>MSQSQRSTADWQRLDAAHHLHPFTDYGELNTKGSRIITRAEGCYLWDSDGNQILDGMAGLWCVNIGYGRKELAEVAYRQMQELPYYNNFFQCSHPPAIELSRLLSEVTPKHMNHVFFTGSGSDSNDTILRMVRYYWKLLGKPYKKVVISRENAYHGSTVAGASLSGMKAMHAQGDLPIPGIEHIEQPYHFGRAPDMDPAEFGRQAAQALERKIDEIGECNVAAFIAEPIQGAGGVIIPPDSYWPEIKRICAERD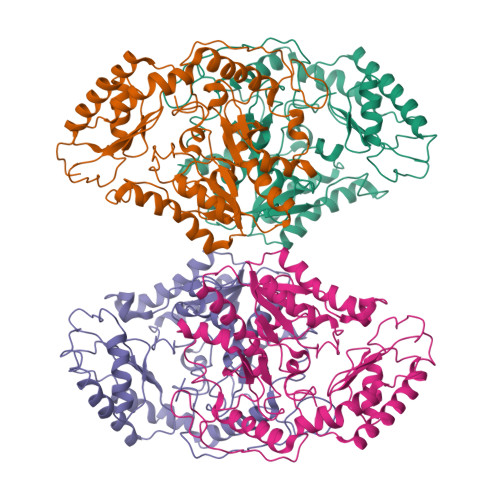ILLIVDEVITGFGRLGTWFGSQYYDLQPDLMPIAKGLSSGYMPIGGVMVSDRVAKVVIEEGGEFFHGYTYSGHPVAAAVAAENIRIMRDEGIIERAGAEIAPYLQARWRELGEHPLVGEARGVGMVAALELVKSKQPLERFEEPGKVGSLCRDLSVKNGLVMRAVGGTMIISPPLVLSREQVDELIDKARRTLDETHKAIGGALEHHHHHH[4x]> EFSEEC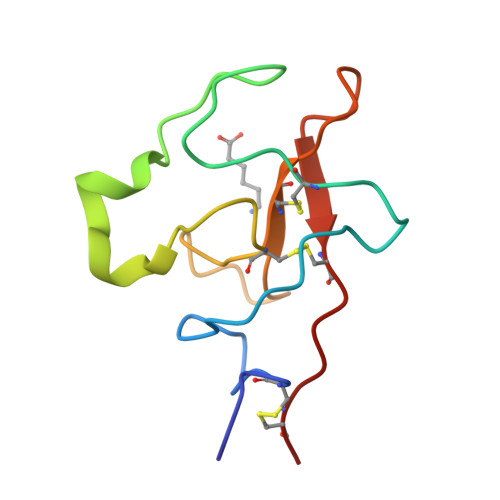MHGSGENYDGKISKTMSGLECQAWDSQSPHAHGYIPSKFPNKNLKKNYCRNPDNDPQGPWCFTTDPNKRWEYCDIPRCA>[2x]MSELARKLLEASTKLQRLNIRLAEALLEAMARLQELNLELVYLAVELTDPKRIRDEIKEVKDKSKEIIRRAEKEIDDAAKESEKILEEAREAISGSGSYLAKLLLKAIAETQDLNLRAAKAFLEAAAKLQELN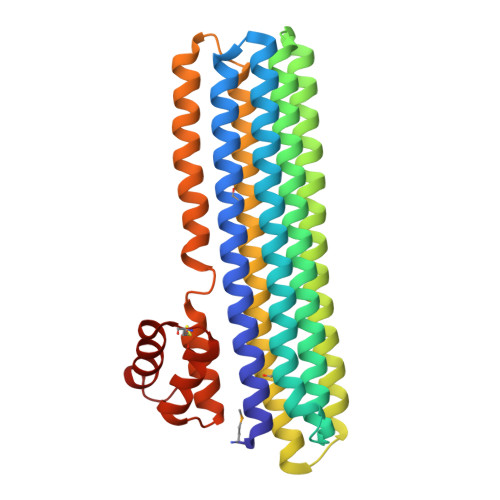IRAVELLVKLYDPATIREALEHAKRRSKEIIDEAERAIRAAKRESERIIEEARRLIEKGSGSGSELARELLRAHAQLQRLNLELLRELLRALAQLQELNLDLLRLASELTDPDEARKAIARSKRESKRIVEDAERGGGTFACRIAAKIAAEFGYSEEQIKELLKNAGCSEDEARDAVEYLRSRPGL>DQPSVGDAFDKYNEAVKVFTQLSSAANCDWPACLSSLSASSAACIAAIGELGLDIPLDLACAATATTSATQACKGCLW[4x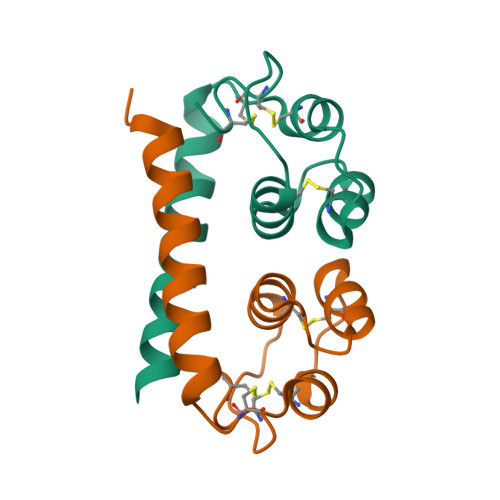]> GAADKGEIRVGNRYQADITDLLKEGEEDGRDQSRLETQVWEAHNPLTDKQIDQFLVVARSVGTFARALDCSSSVRQPSLHMSAAAASRDITLFHAMDTLHKNIYDISKAISALVPQGGPVLCRDEMEEWSASEANLFEEALEKYGKDFTDIQQDFLPWKSLTSIIEYYYMWKTTDRY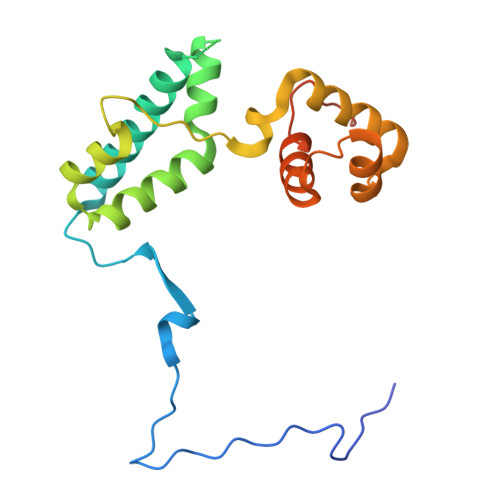VQQKRLKAAEAESKLKQV>[6x]GPGFGGVFVGSFKIINYHLATIEERQSAIYVDWQSDVLVTPIAAHGRHQIARCKCNTGVYYCRHRDKSYPVCF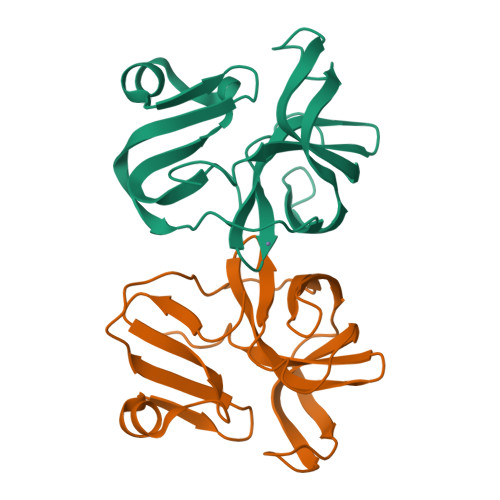EGPGIQWIEQNEYYPARYQTNVLLAAGPAEAGDAGGLLVCPHGVIGLLTAGGGGIVAFTDIRNLLWLDTDAMEQ> ANTLVEDVNICLQACSSLHALSSSLPDDLLQRCVDVCRVQLVHSGTRIRQAFGKLLKSIPLDVVLSNNNHTEIQEISLALRSHMSKAPSNTFHPQDFSDVISFILYGNSHRTGKDNWLERLFYSCQRLDKRDQSTIPRNLLKTDAVLWQWAIWEAAQFTVLSKLRTPLGRAQDTFQTIEGIIRSLAAHTLNPDQDVSQWTTADNDEGHGNNQLRLVLLLQYLENLEKLMYNAYEGCANALTSPPKVIRTFFYTNRQT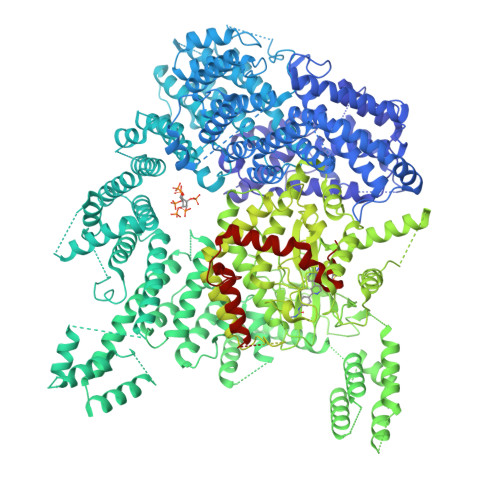CQDWLTRIRLSIMRVGLLAGQPAVTVRHGFDLLTEMKTTSLSQGNELEVTIMMVVEALCELHCPEAIQGIAVWSSSIVGKNLLWINSVAQQAEGRFEKASVEYQEHLCAMTGVDCCISSFDKSVLTLANAGRNSASPKHSLNGESRKTVLSKPTDSSPEVINYLGNKACECYISIADWAAVQEWQNSIHDLKKSTSSTSLNLKADFNYIKSLSSFESGKFVECTEQLELLPGENINLLAGGSKEKINMKKLLPNMLSPDPRELQKSIEVQLLRSSVCLATALNPIEQDQKWQSITENVVKYLKQTSRIAIGPLRLSTLTVSQSLPVLSTLQLYCSSALENTVSNRLSTEDCLIPLFSEALRSCKQHDVRPWMQALRYTMYQNQLLEKIKEQTVPIRSHLMELGLTAAKFARKRGNVSLATRLLAQCSEVQLGKTTTAQDLVQHFKKLSTQGQVDEKWGPELDIEKTKLLYTAGQSTHAMEMLSSCAISFCKSVKAEYAVAKSILTLAKWIQAEWKEISGQLKQVYRAQHQQNFTGLSTLSKNILTLIELPSVNTMEEEYPRIESESTVHIGVGEPDFILGQLYHLSSVQAPEVAKSWAALASWAYRWGRKVVDNASXXXXXXXXXXXXXXXXXXXXXXXXXXXXXXXXXXXXXXXXXXXXXXXXXXXXXXXXXXXXXXXXXXXXXXXXXXXXXXXXXXXXXXXXEGVIKVWRKVVDRIFSLYKLSCSAYFTFLKLNAGQIPLDEDDPRLHLSHRVEQSTDDMIVMATLRLLRLLVKHAGELRQYLEHGLETTPTAPWRGIIPQLFSRLNHPEVYVRQSICNLLCRVAQDSPHLILYPAIVGTISLSSESQASGNKFSTAIPTLLGNIQGEELLVSECEGGSPPASQDSNKDEPKSGLNEDQAMMQDCYSKIVDKLSSANPTMVLQVQMLVAELRRVTVLWDELWLGVLLQQHMYVLXXXXXXXXXXXXXXXXXXXXXXXXXXXXXXXXXXXXXXXXXXXXXXXXXXXXXXXXPHEKWFQDNYGDAIENALEKLKXXXXXXXXXXXXXXXXXXXXXXXXXXXXXXXYILRLEEISPWLAAMTNTEIALPGEVSARDTVTIHSVGGTITILPTKTKPKKLLFLGSDGKSYPYLFKGLEDLHLDERIMQFLSIVNTMFATINRQETPRFHARHYSVTPLGTRSGLIQWVDGATPLFGLYKRWQQREAALQAQKAQDSYQTPQNPGIVPRPSELYYSKIGPALKTVGLSLDVSRRDWPLHVMKAVLEELMEATPPNLLAKELWSSCTTPDEWWRVTQSYARSTAVMSMVGYIIGLGDRHLDNVLIDMTTGEVVHIDYNVCFEKGKSLRVPEKVPFRMTQNIETALGVTGVEGVFRLSCEQVLHIMRRGRETLLTLLEAFVYDPLVDWTAGGEAGFAGAVYGGGGQQAESKQSKREMEREITRSLFSSRVAEIKVNWFKNRDEMLVVLPKLDGSLDEYLSLQEQLTDVEKLQGKLLEEIEFLEGAEGVDHPSHTLQHRYSEHTQLQTQQRAVQEAIQVKLNEFEQWITHYQAAFNNLEATQLASLLQEISTQMDLGPPSYVPATAFLQNAGQAHLISQCEQLEGEVGALLQQRRSVLRGCLEQLHHYATVALQYPKAIFQKHRIEQWKTWMEELICNTTVERCQELYRKYEMQYAPQPPPTVCQFITATEMTLQRYAADINSRLIRQVERLKQEAVTVPVCEDQLKEIERCIKVFLHENGEEGSLSLASVIISALCTLTRRNLMMEGAASSAGEQLVDLTSRDGAWFLEELCSMSGNVTCLVQLLKQCHLVPQDLDIPNPMEASETVHLANGVYTSLQELNSNFRQIIFPEALRCLMKGEYTLESMLHELDGLIEQTTDGVPLQTLVESLQAYLRNAAMGLEEETHAHYIDVARLLHAQYGELIQPRNGSVDETPKMSAGQMLLVAFDGMFAQVETAFSLLVEKLNKMEIPIAWRKIDIIREARSTQVNFFDDDNHRQVLEEIFFLKRLQTIKEFFRLCGTFSKTLSGSSSLEDQNTVNGPVQIVNVKTLFRNSCFSEDQMAKPIKAFTADFVRQLLIGLPNQALGLTLCSFISALGVDIIAQVEAKDFGAESKVSVDDLCKKAVEHNIQIGKFSQLVMNRATVLASSYDTAWKKHDLVRRLETSISSCKTSLQRVQLHIAMFQWQHEDLLINRPQAMSVTPPPRSAILTSMKKKLHTLSQIETSIATVQEKLAALESSIEQRLKWAGGANPALAPVLQDFEATIAERRNLVLKESQRASQVTFLCSNIIHFESLRTRTAEALNLDAALFELIKRCQQMCSFASQFNSSVSELELRLLQRVDTGLEHPIGSSEWLLSAHKQLTQDMSTQRAIQTEKEQQIETVCETIQNLVDNIKTVLTGHNRQLGDVKHLLKAMAKDEEAALADGEDVPYENSVRQFLGEYKSWQDNIQTVLFTLVQAMGQVRSQEHVEMLQEITPTLKELKTQSQSIYNNLVSFASPLVTDATNECSSPTSSATYQPSFAAAVRSNTGQKTQPDVMSQNARKLIQKNLATSADTPPSTVPGTGKSVACSPKKAVRDPKTGKAVQERNSYAVSVWKRVKAKLEGRDVDPNRRMSVAEQVDYVIKEATNLDNLAQLYEGWTAWV> GPHMGNFIITERKKAKEERSNPQTDSMDDLLIRRLTDRNDKEAHLN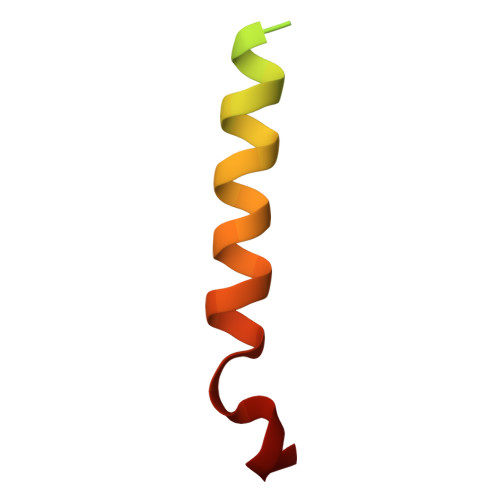ELF>[2x]AAAAAATESDRIAGIFNIPAGIIPTGNVLSTIEVCAHRCIFDFFKQIRSDDNSLYSAQFDILLGTYCNTLNFVRFLELGLSVACICTKFPELAYVRDGVIQFEVQQPMIARDGPHPVDQPVHNYMVKRIHKRSLSAAFAIASEALSLLSNTYVDGTEIDSSLRIRAIQQMARNLRTVLDSFERGTADQLLGVLLEKAPPLSLLSPINKFQPEGHLNRVARAALLSDLKRRVCADMFFMTRHAREPRLISAYLSDMVSCTQPSVMVSRITHTNTRGRQVDGVLVTTATLKRQLLQGILQIDDTAADVPVTYGEMVLNGANLVTALVMGKAVRSLDDVGRHLLDITDPNTLNIPSIPPQSNSDSTTAGLPVNARVPADLVIVGDKLVFLEALERRVYQATRVAYPLIGNIDITFIMPMGVFQANSMDRYTRHAGDFSTV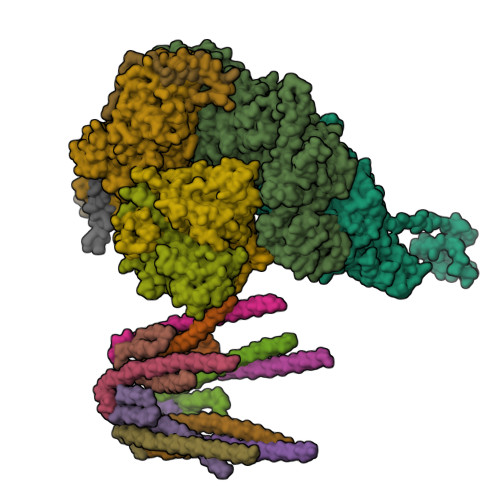SEQDPRQFPPQGIFFYNKDGILTQLTLRDAMGTICHSSLLDVEATLVALRQQHLDRQCYFGVYVAEGTEDTLDVQMGRFMETWADMMPHHPHWVNEHLTILQFIAPSNPRLRFELNPAFDFFVAPGDVDLPGPQRPPEAMPTVNATLRIINGNIPVPLCPISFRDCRGTQLGLGRHTMTPATIKAVKDTFEDRAYPTIFYMLEAVIHGNERNFCALLRLLTQCIRGYWEQSHRVAFVNNFHMLMYITTYLGNGELPEVCINIYRDLLQHVRALRQTITDFTIQGEGHNGETSEALNNILTDDTFIAPILWDCDALIYRDEAARDRLPAIRVSGRNGYQALHFVDMAGHNFQRRDNVLIHGRPVRGDTGQAIPITPHHDREWGILSKIYYYIVIPAFSRGSCCTMGVRYDRLYPALQAVIVPEIPADEEAPTTPEDPRHPLHAHQLVPNSLNVYFHNAHLTVDGDALLTLQELMGDMAERTTAILVSSAPDAGAATATTRNMRIYDGALYHGLIMMAYQAYDETIATGTFFYPVPVNPLFACPEHLASLRGMTNARRVLAKMVPPIPPFLGANHHATIRQPVAYHVTHSKSDFNTLTYSLLGGYFKFTPISLTHQLRTGFHPGIAFTVVRQDRFATEQLLYAERASESYFVGQIQVHHHDAIGGVNFTLTQPRAHVDLGVGYTAVCATAALRCPLTDMGNTAQNLFFSRGGVPMLHDNVTESLRRITASGGRLNPTEPLPIFGGLRPATSAGIARGQASVCEFVAMPVSTDLQYFRTACNPRGRASGMLYMGDRDADIEAIMFDHTQSDVAYTDRATLNPWASQKHSYGDRLYNGTYNLTGASPIYSPCFKFFTPAEVNTNCNTLDRLLMEAKAVASQSSTDTEYQFKRPPGSTEMTQDPCGLFQEAYPPLCSSDAAMLRTAHAGETGADEVHLAQYLIRDASPLRGCLPL;> AMPFEIEVLLPGELSPAETSALQKCEGKIITFSTLRHRASLVDIALSSYYINGAPPDTLSLLEAYRMRFAAVITRVIPGKLLAHAIGVGTPTPGLFIQNTSPVDLCNGDYICLLPPVFGSADSIRLDSVGLEIVFPLTIPQTLMREIIAKVVARAVEDLNPDPDLNVLYYNGARLSLVADVQQLASDAAIRTLVLNLMFSINEGCLLILALIPRLLALGYVNALLQMQSVTREAAQLIHPEAPMLMRRLPIYETISSWISTSSRLGDTLGTRAILRVCVFDGPSTVHPGDRTAVIQV;> AMPFEIEVLLPGEISPAETSALQKCEGKIITFSTLRHRASLVDIALSSYYINGAPPDTLSLLEAYRMRFAAVITRVIPGKLLAHAIGVGTPTPGLFIQNTSPVDLCNGDYICLLPPVFGSADEIRLDSVGLEIVFPLTIPQTLMREIIAKVVARAVERTAAGRTPGELPGADVICYNGRRYELETNLQHRDGSDAAIRTLVLNLMFSINEGTTLILTLITRLLVQGAHDGYVNLLIQTANCVRETGQPMPRIQDGHRRFPIYEAISSWISTSSRLGDTLGTRAILRVCVFDGPSTVHPGDRTAVIQV;> TTQLIQQVSLTDFFRPDIEHAGSTVLILRHPTDLPHLARHRAPPGRQTERLAEAWGQLLEASESGCARAYVTSLSFIAACRAEEYTDKQAAEANRTAIVSAYGCSRMGARLIRFSECLRAMVQCHVFPHRFISFFGSLLEYTIQDNLCNITAVAKGPQEAARTDKTSTRRVTANIPACVFWDVDKDLHLSADGLKHVFLVFVYTQRRQREGVRLHLALSQLNEQCFGRGIGFLLGARICMYAAYTLIGTIPSESVRYTRRMERFGGYNVPTIWLEGVVWGGTNTWNECY;> MNAHLANEVQYDLGHPSSLVHVIISSECLAAAGIPLAALMRANFQVEIQTRAHATGDCTPWCTAFAAYVPADAVGELLAPVVPAHPGLLPRASSAGGLFVSLPVVCDAQGVYDPYAVAALRLAWGSGASCARVILFSYDELVPPNTRYAADSTRIMRVCRHLCRYVALLGAAAPPAAKEAAAHLSMGLPPISPEEQLTAPGGDTTAAQDVSIAQENEEILALVQRRSLVEWLDRGWEALAGGDRPDWLWSRRSISVVLRHHYGTKQRFVVVSYENSVAWGGRRARPPLLSSALATALTEACAAERVVRPHQLSPAGQAELLLRFPALEVPLRHPRPVLPPFDIAAEVAFTARIHLACLRALGQAIRAALQGGPRISQRLRYDFGPDQRAWLGEVTRRFPILLENLMRAVEGTAPDAFFHTAYALAVLAHLGGRVVPLGDDLPARFADSDGHYVFDYYSTSGDTLRLNNRPIAVAMDEQSKCRFMEAPRRVCEQYLPGESYAYLCLGFNRRLCGIVVFPGGFAFTINIAAYLSLSDPVARAAVLRFCRKVS;>[2x]MDPYCPFDALDVWEHRRFIVADSRNFITPEFPRDFWMSPVFNLPRETAAEQVVVLQAQRTAAAAALENAAMQAAELPVDIERRLRPIERNVHEI;>[2x]QRTGRSALAVLIRACYRLQQQLQRTRRALLHHSDAVLTSLHHVRMLL> GSMNHIHEHLKLVPVDKIDLHETFEPLRLEKTKSSIEADDFIRHPILVTAMQHGRYMVIDGVHRYTSLKALGCKKVPVQEIHETQYSISTWQHKVPFGVWWETLQQEHRLPWTTETRQEAPFITMCHGDTEQYLYTKDLGEAHFQVWEKVVASYSGCCSVERIAQGTYPCLSQQD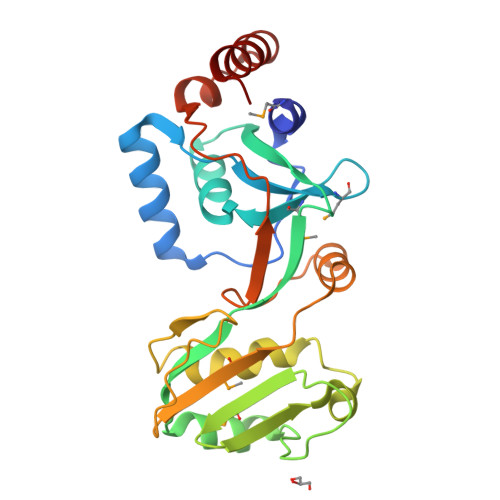VLMKYQPLSYKEIEAVVHKGETVPAGVTRFNISGRCLNLQVPLALLKQDDDVEQLRNWKQFLADKFA The P. infestans RXLR-type effector PexRD54 (PITG_09316) perturbs host-selective autophagy for the benefit of the pathogen via interaction with ATG8CL. Recently, a P. infestans RXLR effector, PexRD54, which contains an AIM sequence Trp-Glu-Ile-Val “WEIV” positioned at the C terminus (residues 378–381), was identified. It was shown that PexRD54 specifically interacts with a member of the ATG8 family of proteins from potato, ATG8CL, in vitro and in planta. In plant cells, PexRD54 activates selective autophagy by increasing the number of ATG8CL-containing autophagosomes and stabilizing ATG8CL.

To discover the molecular architecture of PexRD54, we determined the crystal structure of the effector domain of this protein (residues Val-92 to Val-381) at 2.90 Å resolution. Although PexRD54 could be crystallized alone, the crystal that gave rise to the best x-ray dataset was obtained from a sample including both PexRD54 and ATG8CL after co-expression in E. coli (see under “Experimental Procedures”). Although SDS-polyacrylamide gel analysis of dissolved crystals showed that both proteins were present in these crystals, no electron density for ATG8CL was observed. Five N-terminal residues (92–96), the residues in two loops (248–250 and 331–334), and 11 C-terminal residues (371–381), which include the AIM motif, were not included in the final model due to poor electron density in these regions. The structure of PexRD54 includes 16 α-helices. Our structural analysis revealed that PexRD54 includes five tandem WY domains that pack to form an elongated molecule. This is a conformation not yet observed for RXLR effectors with multiple WY domains. The WY domain is a conserved structural unit consisting of three α-helices and two characteristic hydrophobic amino acids, frequently W (Trp) and Y (Tyr), which contribute to a stable hydrophobic core. Interestingly, in PexRD54, the C-terminal helices of WY-1, WY-3, and WY-4 are positioned such that they also serve as N-terminal helical extensions to WY-2, WY-4, and WY-5 to build four-helical bundles as observed in AVR3a4 (42), AVR3a11, and ATR1. Finally, PexRD54:WY-3 does not have an N-terminal helix and does not form a four helical bundle. This correlates with a significant kink in the PexRD54 structure between WY-2 and WY-3.

> GPVTSSLSAEEAQLKVWIQSQIHPRELFGVLSLGKRAAKLDDNPDFVQWLRLVKDFRANNGNQAFSDLDIYYLLLKTNSPEQLKLLFETLRHTPGMTKIGASMEKSLSGNWIRKALEQDTYPTIVYNTLRLKDAGTKLDDTPMFRQWLEYVEKYWNKNAGAFFGDTQMLTLFQKTMTEEEDIIKLVHMLRNNPGMKSHADKLERYLLLTSESSHKTMADVWLKARETPEEVFRILRLAEKQTAAADDNRMLNLWLRYTQTYRDKIDKNAFSDAEALQFFRKAKPLDFDWEIV> UGCCUGGCGGCCGUAGCGCGGUGGUCCCACCUGACCCCAUGCCGAACUCAGAAGUGAAACGC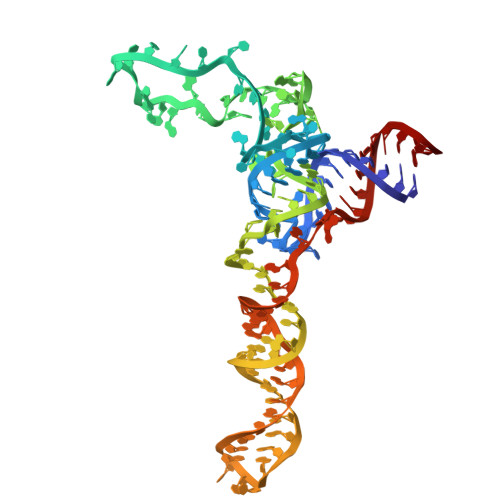CGUAGCGCCGAUGGUAGUGUGGGGUCUCCCCAUGCGAGAGUAGGGAACUGCCAGGCAU>[3x]MVYEAITAGGFGSQPFILAYIITAMISGLLFLYLPRKLDVPQKFGIIHFFIVVWSGLMYTNFLNQSFLSDYAWYMDWMVSTPLILLALGL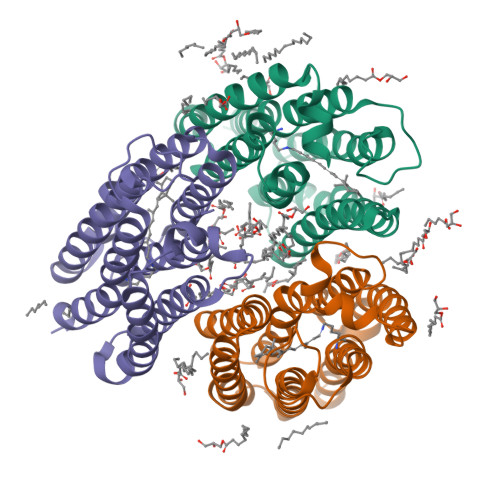TAFHGADTKRYDLLGALLGAEFTLVITGLLAQAQGSITPYYVGVLLLLGVVYLLAKPFREIAEESSDGLARAYKILAGYIGIFFLSYPTVWYISGIDALPGSLNILDPTQTSIALVVLPFFCKQVYGFLDMYLIHKAELEHH>MKGFAMLGINKLGWIEKERPVAGSYDAIVRPLAVSPCTSDIHTVFEGALGDRKNMILGHEAVGEVVEVGSEVKDFKPGDRVIVPCTTPDWRSLEVQAGFQQHSNGMLAGWKFSNFKDGVFGEYFHVNDADMNLAILPKDMPLENAVMITDMMTTGFHGAELADIQMGSSVVVIGIGAVGL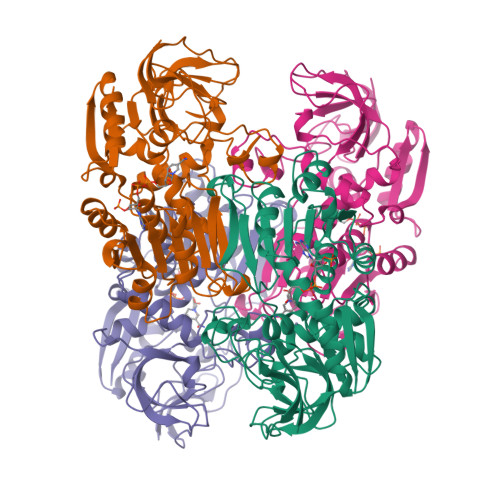MGIAGAKLRGAGRIIGVGSRPICVEAAKFYGATDILNYKNGHIVDQVMKLTNGKGVDRVIMAGGGSETLSQAVSMVKPGGIISNINYHGSGDALLIPRVEWGCGMAHKTIKGGLCPGGRLRAEMLRDMVVYNRVDLSKLVTHVYHGFDHIEEALLLMKDKPKDLIKAVVIL[4x]Pex15 and its homologs are tail-anchored proteins with poor sequence conservation and no known structure, yet they share a common function in recruiting the Pex1/Pex6 AAA-ATPase motor to the peroxisome membrane. Here we show that Pex15 inhibits the ATPase activity of Pex1/Pex6 because its cytosolic portion is recognized as a substrate, engaged by the pore loops, and completely unfolded by the AAA motor. Pex1/Pex6 then unfolds Pex15 and any N-terminally fused proteins by processive threading through the central pore in an ATP-hydrolysis-dependent manner. Based on these findings, the current model is that Pex15 recruits Pex1/Pex6 to the peroxisomal membrane and directly links it to Pex5/Pex14 and potentially other Pex proteins.

Using limited proteolysis on the cytosolic domain of yeast Pex15, we determined that Pex15 consists of a stable core region (aa 43–253) with disordered N-terminal and C-terminal tails. Without these disordered regions, the 25 kDa core was readily amenable to crystallization, and we solved its structure at 1.55 Å resolution. The core consists of 12 α-helices that fold into a compact, curved structure stabilized by a network of hydrophobic interactions. The crystal structure of Pex15 shows a single domain that we predicted would unfold cooperatively in one step. Consistently, measurement of the denaturant-induced equilibrium unfolding by circular dichroism exhibited a single transition with no indication of stable intermediates. In order to measure the unfolding of Pex15 by Pex1/Pex6 with higher throughput, we took advantage of the observation that all of the cysteine residues of Pex15 reside within the folded core and are inaccessible to solvent. Guided by its curved shape and the orientation of its longest helix, the core-domain structure of Pex15 was docked into the difference density above the Pex6 N-terminal domains. Building upon the atomic model for Pex1/Pex6 proposed by Blok et al., this placement suggests that Pex15’s N-terminus binds between the N1 and N2 domains of Pex6. We note that the 42 N-terminal residues of Pex15 that are not included in the crystal structure can be accommodated in the additional, unfilled density at the contact sites between Pex15 and Pex6.

> MSEVFQECVNLFIKRDIKDCLEKMSEVGFIDITVFKSNPMILDLFVSACDIMPSFTKLGLTLQSEILNIFTLDTPQCIETRKIILGDLSKLLVINKFFRCCIKVIQFNLTDHTEQEEKTLELESIMSDFIFVYITKMRTTIDVVGLQELIEIFIFQVKVKLHHKKPSPNMYWALCKTLPKLSPTLKGLYLSKDVSIEDAILNSIDNKIQKDKLEVLFQ> GTSSE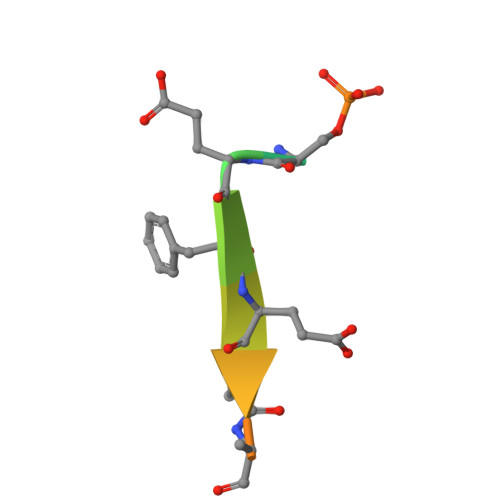FEVVTPEE>[2x]ENLYFQGMLEGDLVSKMLRAVLQSHKNGVALPRLQGEYRSLTGDWIPFKQLGFPTLEA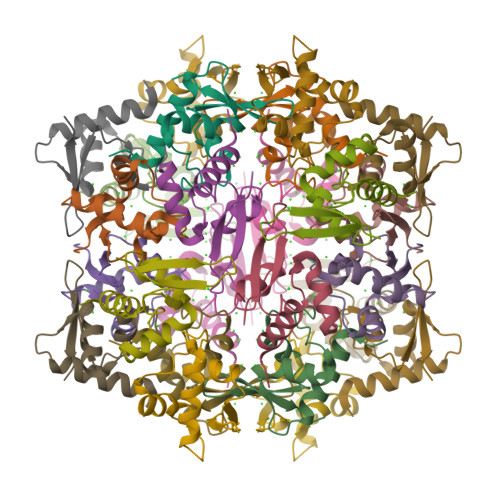YLRSVPAVVRIETSRSGEITCYAMACTETAR>[4x]MGSSHHHHHHGSLDTNAVKEPEPALPSAASRGRRTKNWWEPMFDANAPASFSVSDWNFSNNRGPRCTLFLAEKMPDATTLVVKDIDFQDCDFQGTFERKIVFKDCKFTRCDFGLSTFSRTKFSGCSFYASSFTQCTLENCEFRNCKYEKIFYSGNETQI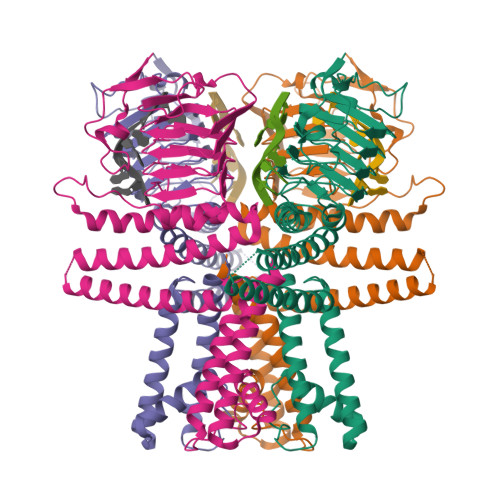PRTLIAEPYQFLFGACATVDSVPQGKSRFEQRARFEETRSTIARALLANLHSEGSEDTYYAAVKASTLSENRARIARALIKINSSASKGKSIISRAVSFLTGFASAISAVVGMLILLVMGSLNGWGSSISRAMLVGVVAISCVAYRYHYRFNLPPEDAMVKATEIFFLFGYTNYAKMGQEDFHLVFSNALLGLFWYAIAIPTISNRLTRARG(2S)-hexane-1,2-diol | C6 H14 O2 | 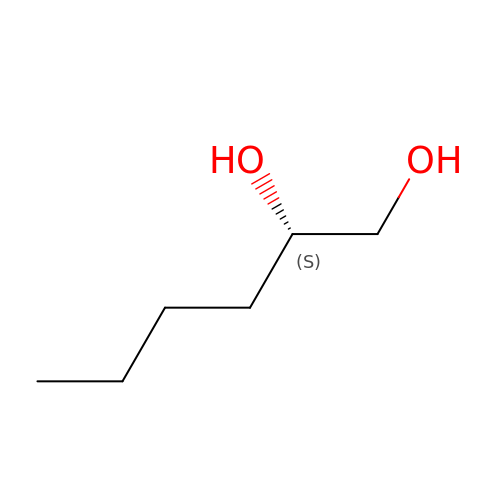FHKSXSQHXQEMOK-LURJTMIESA-N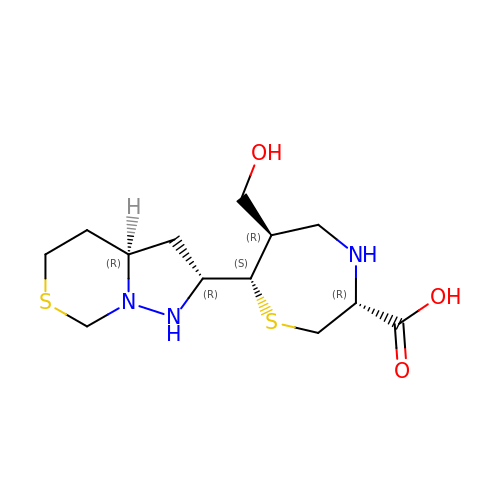(3R,6R,7S)-7-[(2R,3aR)-hexahydropyrazolo[1,5-c][1,3]thiazin-2-yl]-6-(hydroxymethyl)-1,4-thiazepane-3-carboxylic acid | C13 H23 N3 O3 S2 | BYDOKGBTKWANQM-LVEVGFFFSA-N>MGSSHHHHHHGSGENLYFQSNQPLKIVVPFSAGGTADVLPRLVAEKIRADYAGGVIIENKPGAGGNIGADLVFRAPPDGMTVLASPPGPIAINHNLYQKLSFDPTRWVPVTILATVPNVLVINPKLPVKSLGEFIAYAKANPKKVTVATQGDGSTSHLTAAMFMQLTGTELTVIPYKGTAPALIDLIGGNVDVFFDNISSSATYHQAGKVRILAVADEQRSQILPQVPTFAEQQWPAMQAVTFFSVVAPPGTSAEIAQKLQKQMALALSSNDIRKHFQEQGAVPCGWDPSKTAQFIRQETEKWKKVLKAANVKL[6x]

In this study, we characterised the TphC SBP that is a key component in the cellular uptake of TPA, the breakdown product of PET plastic. TphC belongs to the TTT family in Commamonas sp. strain E6 and through biochemical and structural analysis, the ligand-binding properties and 3D structure were determined in both open and ligand-bound closed forms. As with the tripartite ATP-independent periplasmic (TRAP) class of SBP-dependent transporters, they are symporter proteins driven by an electrochemical ion-gradient, rather than ATP as per the SBP-dependent class of ABC transporters. Here, we report the biochemical and structural characterisation of TphC in both open and TPA-bound closed conformations. This analysis demonstrates the narrow ligand specificity of TphC towards aromatic para-substituted dicarboxylates, such as TPA and closely related analogues.

In order to understand the open structure of TphC, we sought to crystalise TphC alone. A Crystal structure of TphC is shown in ribbon representation (α-helices red, β-strands green), the structure is comprised of two domains with a large solvent accessible cleft located at the domain interface. Residues (P28-D37, PFSAGGTAD) map to the motif [P∗-F-X-A-G∗-G∗-X-X-D∗] which is highly conserved in TTT-SBPs (conserved residues underlined). Superposition of the open and closed TphC structures highlights an ~36° closure between the two domains upon TPA binding. Overlaying the open and closed TphC structures indicates the movement of the upper domain (α4–α6). TphC shows a 36.3° closure angle, whereas previously resolved apo- and ligand-bound structures of Bug27 reported a closure angle of 24.7°51 and other periplasmic binding proteins show closure angles ranging from 15° to 60°58.>[4x]MLKAVILI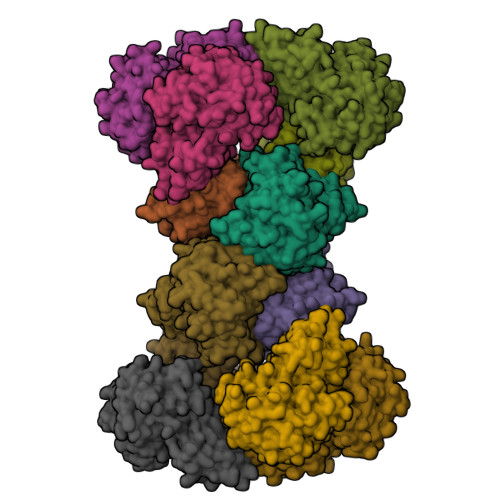GGPQKGTRFRPLSFEVPKPLFPVAGVPMIQHHIEACAQVPGMQEILLIGFYQPDEPLTQFLEAAQQEFNLPVRYLQEFAPLGTGGGLYHFRDQILAGSPEAFFVLNADVCSDFPLSAMLEAHRRQRHPFLLLGTTANRTQSLNYGCIVENPQTHEVLHYVEKPSTFISDIINCGIYLFSPEALKPLRDVFQRNQQDGQLEDSPGLWPGAGTIRLEQDVFSALAGQGQIYVHLTDGIWSQIKSAGSALYASRLYLSRYQDTHPERLAKHTPGGPWIRGNVYIHPTAKVAPSAVLGPNVSIGKGVTVGEGVRLRESIVLHGATLQEHTCVLHSIVGWGSTVGRWARVEGTPSDPNPNDPRARMDSESLFKDGKLLPAITILGCRVRIPAEVLILNSIVLPHKELSRSFTNQIIL;>[8x]MKALILVGGYGTRLRPLTLSTPKPLVDFCNKPILLHQVEALAAAGVDHVILAVSYMSQVLEKEMKAQEQRLGIRISMSHEEEPLGTAGPLALARDLLSETADPFFVLNSDVICDFPFQAMVQFHRHHGQEGSILVTKVEEPSKYGVVVCEADTGRIHRFVEKPQVFVSNKINAGMYILSPAVLQRIQLQPTSIEKEVFPIMAKEGQLYAMELQGFWMDIGQPKDFLTGMCLFLQSLRQKQPERLCSGPGIVGNVLVDPSARIGQNCSIGPNVSLGPGVVVEDGVCIRRCTVLRDARIRSHSWLESCIVGWRCRVGQWVRMENVTVLGEDVIVNDELYLNGASVLPHKSIGESVPEPRIIM6-(1H-Indol-4-yl)-4-(5-{[4-(1-methylethyl)-1-piperazinyl]methyl}-1,3-oxazol-2-yl)-1H-indazole 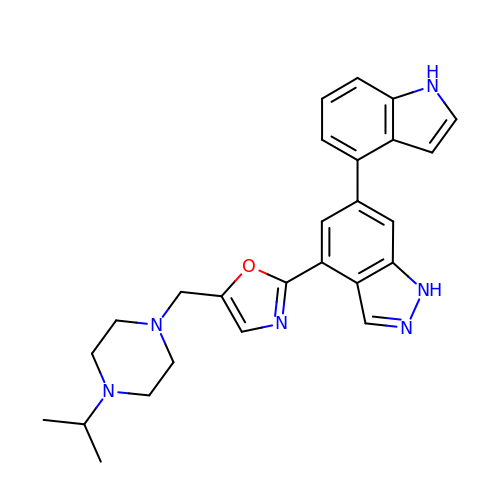| C26 H28 N6 O | MCIDWGZGWVSZMK-UHFFFAOYSA-N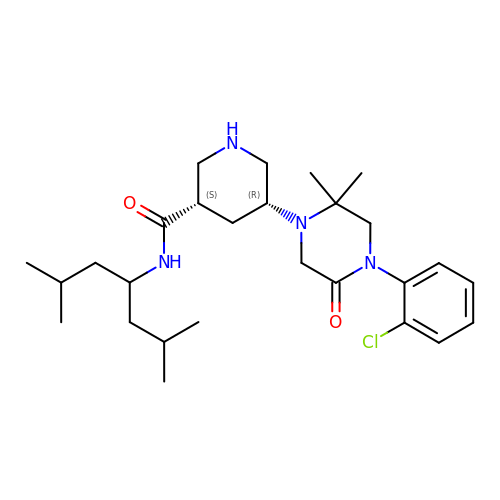(3S,5R)-5-[4-(2-chlorophenyl)-2,2-dimethyl-5-oxopiperazin-1-yl]-N-(2,6-dimethylheptan-4-yl)piperidine-3-carboxamide | C27 H43 Cl N4 O2 | VVEBLTKFUFYNOR-RBBKRZOGSA-N>[2x]GSHMTARTPDAEPPLLTPAEVATMFRVDPKTVTRWAKAGKLTSIRTMGGHRRYREAEVRALMAGIPQQRSEA

Like BldD and BldO, BldC acts as a repressor to sustain vegetative growth, and so deletion of bldC causes the premature onset of sporulation. bldC encodes a 68-residue protein that is predicted to contain a winged helix-turn-helix (wHTH) motif, suggesting it may be involved in DNA binding. While BldC appears to contain a MerR-like wHTH, it is to date, the only known MerR-like protein that consists entirely of a wHTH with no obvious effector or oligomerization domain. Using a battery of structural, biochemical, and in vivo approaches, we show here that BldC functions as a pleotropic regulator of Streptomyces development by employing a unique mode of DNA binding for a transcription factor that involves asymmetric head-to-tail oligomerization on DNA direct repeats of varying number with concomitant distortion of the DNA.

Thus, to deduce the molecular mechanism underlying DNA binding and recognition by BldC, we determined the structure of S. coelicolor BldC bound to a 22 bp double-stranded DNA based on the optimized whiI binding site (whiI opt). The structure was solved by single wavelength anomalous diffraction (SAD) using data collected from a selenomethionine-substituted BldC(L43M-L58M)-whiI opt DNA crystal (WT BldC-whiI opt produced the same crystals) and refined to Rwork/Rfree values of 22.3%/26.8% to 3.28 Å resolution. Notably, the structure reveals that BldC forms a head to tail (head-tail) dimer on the DNA whereby each BldC protomer binds to a 9 bp direct repeat with the recognition helix of the HTH motif interacting in the major groove and the wing in the minor groove. Formation of the head-tail BldC dimer buries ~600 Å2 of protein surface from solvent. The oligomer interface is largely hydrophobic with residues Phe21, Val23, and Trp31 packing against the side chains of Leu11′, Ile 40′, Thr42′, Leu43′, and Gly44′ (where ′ indicates the other subunit of the DNA-stabilized dimer). Hydrogen bonds/electrostatic contacts between the side chains of Arg22 and Glu16′ help fasten the two subunits together. The head-tail binding of the two BldC protomers bends the whiI site by ~50°. However, the minor and major groove widths are significantly distorted: the wing-bound, AT-rich minor groove has an average width of 9.3 Å (compared to 12.0 Å for B-DNA) whereas the minor groove outside this region is widened significantly (14.5 Å). However, despite the low resolution, the electron density for the Arg30 side chain is clear and reveals that it provides highly specific, bidentate hydrogen bonds to Gua2′ and Gua11′. Thus, the analysis of the BldC-whiI opt structure indicates that there are two main DNA elements specifically recognized by BldC; an AT-rich region and a C-G, 4 base pairs downstream from the AT-rich region, which is recognized by Arg30.3-chloro-N-{4-[1-(propylcarbamoyl)cyclobutyl]phenyl}benzamide | C21 H23 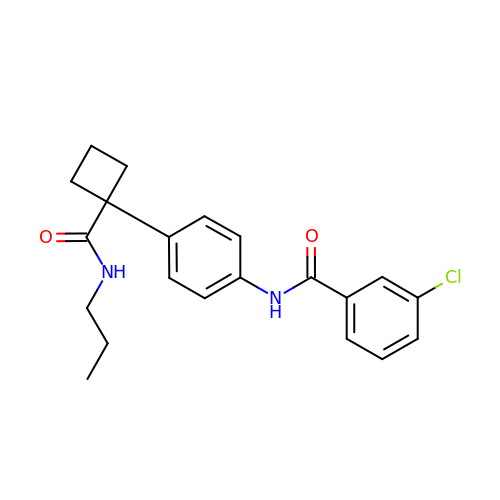Cl N2 O2 | UIZYWUYIFDOVIY-UHFFFAOYSA-N>[2x]SGWDEFTKHVTSECLGWMRQQRAEMDMVAWGVDLASVEQHINSHRGIHNSIGDYRWQLDKIKADLREKSAIYQLEEEYENLLKASFERMDHLRQLQNIIQATSREIMWINDCEEEELLYDWSDKNTNIAQKQEAFSIRMSQLEVKEKELNKLKQESDQLVLNQHPASDKIEAYMDTLQTQWSWILQITKCIDVHLKENAAYFQFFEEAQSTE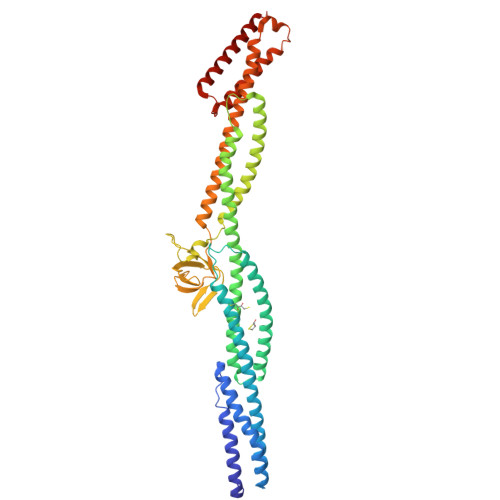AYLKGLQDSIRKKYPCDKNMPLQHLLEQIKELEKEREKILEYKRQVQNLVNKSKKIVQLKPRNPDYRSNKPIILRALCDYKQDQKIVHKGDECILKDNNERSKWYVTGPGGVDMLVPSVGLIIPPPNPLAVDLSCKIEQYYEAILALWNQLYINMKSLVSWHYCMIDIEKIRAMTIAKLKTMRQEDYMKTIADLELHYQEFIRNSQGSEMFGDDDKRKIQSQFTDAQKHYQTLVIQLP>ADASDWLNRLAEADRQNSFQGTFVYERNGSFSTHEIWHRVESDGAVR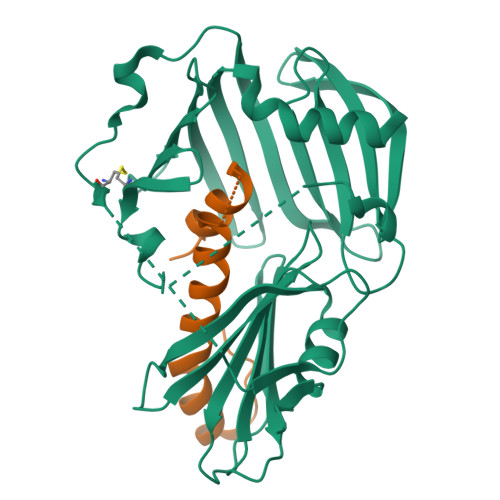ERLLQLDGARQEVVRVDGRTQCISGGLADQLADAQLWPVRKFDPSQLASWYDLRLVGESRVAGRPAVVLAVTPRDQHRYGFELHLDRDTGLPLKSLLLNEKGQLLERFQFTQLNTGAAPAEDQLQAGAECQVVGPAKADGEKTVAWRSEWLPPGFTLTRSFMRRSPVTPDPVACLTYGDGLARFSVFIEPLHGAMVGDARSQLGPTVVVSKRLQTDDGGQMVTVVGEVPLGTAERVALSIRPEAAAQK[2x];>[2x]YNQNDALPQMAQQGTTPQIALPQVKGPAVLAGYSEEQGAPQVITNSSSSDTRWHEQRLPIYLRQHVQQSAVSGTESALPYARAASLENR(4R)-4-(3-HYDROXYPHENYL)-N,N,7,8-TETRAMETHYL-3,4-DIHYDROISOQUINOLINE-2(1H)-CARBOXAMIDE 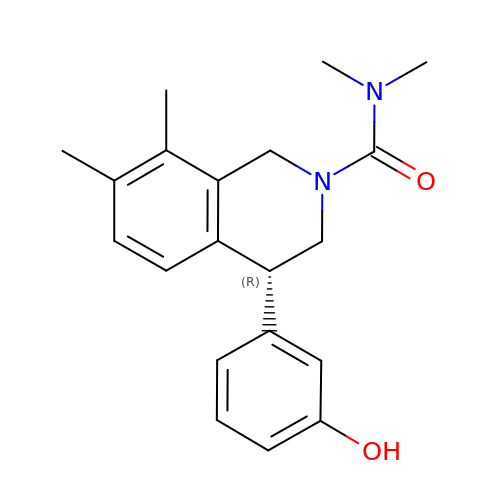| C20 H24 N2 O2 | HPVCRUIDFODATB-LJQANCHMSA-N>[2x]MTVELCGRWDARDVAGGRYRVINNVWGAETAQCIEVGLETGNFTITRADHDNGNNVAA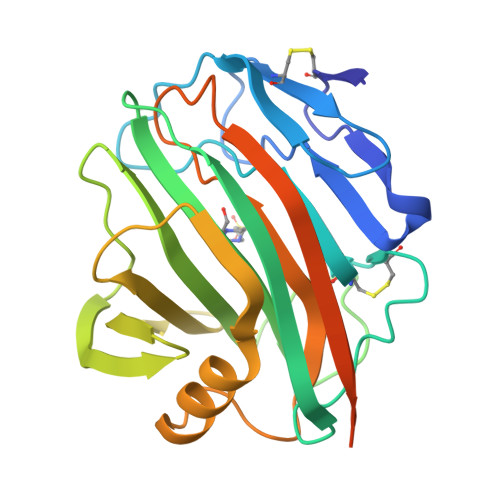YPAIYFGCHWGACTSNSGLPRRVQELSDVRTSWTLTPITTGRWNAAYDIWFSPVTNSGNGYSGGAELMIWLNWNGGVMPGGSRVATVELAGATWEVWYADWDWNYIAYRRTTPTTSVSELDLKAFIDDAVARGYIRPEWYLHAVETGFELWEGGAGLRSADFSVTVQKLAAALEIKRASQPELAPEDPEDVEHHHHHH> SNAKNTMPLVIAYNNAPEDDKIQKLFYLQKINYLLNKTQLNDDLFDWINDAEEGGWLNELAKFSINPNASFFLKGMQFAKAITEEIKNKPEINSSEVNIYHLMQERDQLLKEVEFEKCATRYAEINFLLNELALNDKKTKEIVERQTEILRLVAPKIKAIKGESIDNLPVIPSYKTKELGNHVNNFNFKFTMSGWEAPFVFRVEDRHELGKEQELHSYGVSKYFIEDYSVFMMRFKAEDGSTVYKPVILSQFANQNNLEEIAKQLKDGSPKNIAPRIGYYFVQLTDFCLKLIETHNYHPDIKLNNFLVHNNRVLVSDRKTFTTNDNPLASEILTSPLFAPDEFLKCLLFNKEGDPVGYNRNALWKRMNMPQFMAYQLGMALKQFLILTQLDELPDDFR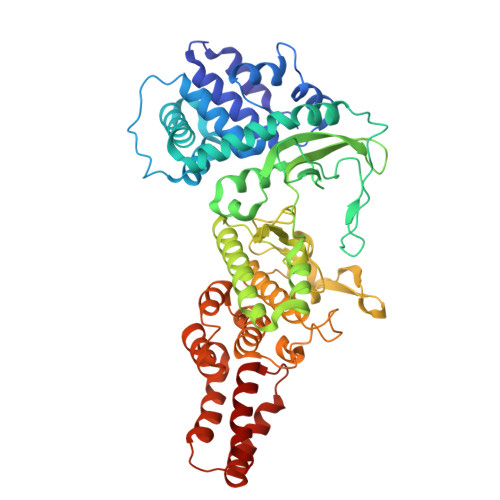NPDHSAVSHFKTPSRQIINLSLLVQELTRLDPDKRMTIKQFQTLLNFKNLPPDAFYQKVEEVFPSSQLGIAEDIEALNKVLNSDLKGEALLKQANPVFTKLSKYDPKETRLTRLAEKLAIRCFNN>MTSMASLFSFTSPAVKRLLGWKQGDEEEKWAEKAVDALVKKLKKKKGAMEELEKALSSPGQPSKCVTIPRSLDGRLQVSHRKGLPHVIYCRVWRWPDLQSHHELKPLDICEFP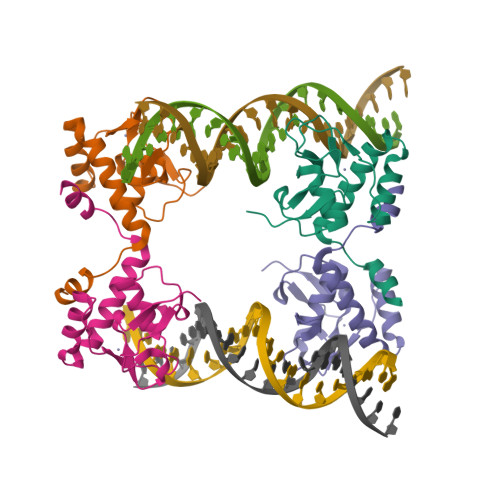FGSKQKEVCINPYHYKRVESPVLPPVLVPRLEHHHHH[4x]2-azanyl-~{N}-[2-bromanyl-5-[4-[3-(dimethylamino)propylsulfonyl]piperazin-1-yl]phenyl]-1,3-oxazole-4-carboxamide | C19 H27 Br N6 O4 S | 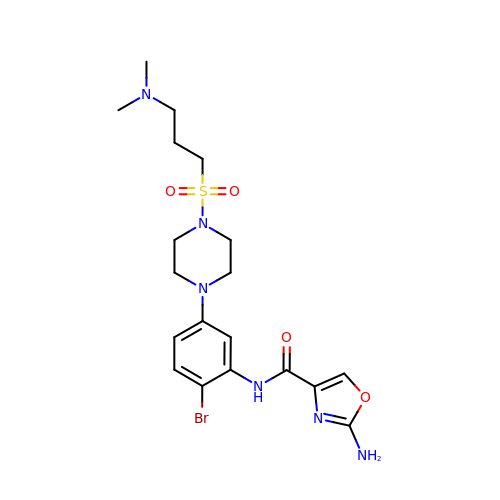GTJMWLKWMPRNKA-UHFFFAOYSA-N>[4x]GSPSRKFYWKARSQMCEVKGWVPTHRGFPWGPELPGDLILSRRAYVSCDLTSCFKFFIAYGLSANQHLLNTSMEWEESLYKTPIGSANTLSTSEMILPGRSSSACFDGLKWTVLVSNGRDRNSFIMIKYGEEITDTFSASRGGPLRLPNSECICVEGSCFVLVSDGPNVNQSVHRIYELQNGTVQRWKQLNTTGINFEYS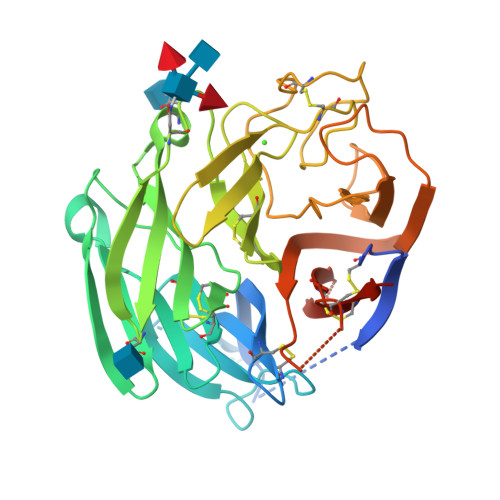TCYTINNLIKCTGTNLWNDAKRPLLRFTKDLNYQIVEPCNGAPTDFPRGGLTTPSCKMAQEKGEGGIQGFILDEKPAWTSKTKTELSQNGFVLEQIPDGIESEGTVSLSYELFSNKRTGRSGFFQPKGDLISECQRVCFWLEIEDQTVGLGMIQELSTFCGINSPVQNINWDS> MLVEDLLKNNYLITPSAYYLLSDHYKKAFTLAELIKFAKNRGTFVVDSNLAREFLAEKGIISSGIVYGDYGVPIAYVADETPEEEKAYSTYSDLVIAPKEGFHYRAKEIPDEWELAFDVKNVKFEVPKVKNAQSKEGEVIIQAYSSYFKSRLKKMRRIFRENPEIGTIVDIAKLSYVREDDVTIIGLVNEKRETRKGYLFEIEDATGRIKVFIGSDKEGANEAYSTIMPDSVVAFRGTPGKGIFFANRVFLPDVPKFKRSKPPLEEKVYAILLSDIHVGSNKFCEEAFIKFLEWLNGEVNSRTEEELVSRIKYIIIGGDVVDGVGIYPGQYNELAIPDIFDQYEALANLLKQVPDHITMFIGPGNHDAARTALPQPGFYEEYAKPLYKLKNAVIISNPAVIRLHGRDFLVAHGRGIEDVVDFVPNRSHHRPAEAMVELLKLRHIAPTFGNKVPIAPDPEDTLVIESVPDLFQAGHVHVMQYKTYNGVFVINTGTWQAQTEFQKMVNIIPTPARVPIIDVETARLRAVVRFDQFCEGV;> MSEEIYSPEMKAYFESLQREIDRAYAIARKARAQGKDPSFDVEVPQATDMAGRVESLVGPPGVAERIRELVKEYGKEIAALKVVDEIIEGKFGDLGSKEKYAEQAVRTALAILTEGIVSAPLEGIADVKIKRNEWADGSEYLALYYAGPIRSSGGTAQALSVLVGDYVRRKLGLDRFKPSDEHIERMVEEVDLYHRAVTRLQYHPEADEVRLAMRNIPIEITGEETDKVEVSHRNVPGVETNHLRGGAILVLAEGVLQKAKKLVKYIDKMGIEGWDWIKEFVEAKEKGKSSEENKDESKAEDTGTESVAEKKENVEKGFYYELYEKFRANIAPNKKYTKEIIGGRPLFAEPSTNGGFRLRYGRSRVSGFATWSVNPATMLILDEFIAIGTQMKTERPGKGCIVTPATTVEGPIVRLKNGSVVRVDDYETALKVRNEVDEILYVGDALVNFGDFVENNQTLLPANYVEEWWVQELVQAIKDLYEVELQPFAENDREAVEEAAEYLEVDPDFLWNLLKDPLRVKPDVETAIHLSTVLDIPFHPYYTLYWNTLQPEEVEELQKALLGAQIEWAEFRKNRFAKKVVLENDKNIKRYLELLGLPHRLERVEKKRKVIVVEYPWSAALLTPLGNLEWEFKAKPFYTVIDIINENNRIKLRDRGISWIGARMGRPEKAKERKMKPPVQVLFPIGLAGGQSRDIKKAAEEGKTARVEIAFFKCPKCGHVGPEHLCPVCGTRKELLWHCPKCGADYPESDAKDFNYRCPKCDVELKPYAEREIKPADLLRQAMDNVKVYGIDRLKGVKGMTSGYKMAEPLEKGLLRVKNDVYVFKDGTIRFDATDAPITHFKPKEIGTSVEKLRELGYTHDFEGKPLERDDQILELKVQDVILPYEAGRYLLKVARFIDDLLEKFYGLPRFYNAEKMEDLVGHLVIGLAPHTSAGIIGRIIGFSDVLVGYAHPYYHAAKRRNCDGDEDAVMLLLDALLNFSKYYLPEKRGGKMDAPLVVTTRLDPREVDSEVHNMDVVRYYPLEFYKATYELKSPKEVKVIERVEDRLGKPEMYEGIKFTHDTDDIGLGPKMSLYKQLGDMEEKVARQLALAERIRAVDEHHVAETIINSHLVPDLRGNLRSFTRQEFRCVKCNTKYRRPPLTGKCPKCGGKIVLTVSKGAIEKYLPTAKMLVTKYRVKDYTRQRICITEKDIKTLFENVFPEKQRTLMGFSADICEKMVKERTGHSNGKNGYLDEFNGKNGKASKKSGSLASKLSGKGKEPSKKKESAKPKRSEKVKNLTSFEAAAKNEQARGTAGNAKKAESEKPKRKKRKGISLDEFFGS;>MPFEVVFDGAKEFADLIATASNLIDEAAFKFTEEGISMRAMDPSRVVLIDLNLPESIFSKYEVEEPETIGINMDQFKKILKRGKAKDTLILRKGDENFLEITFEGTAKRTFRLPLIDVEELELELPELPFTAKVVLLGEVLKEGIKDASLVSDAIKFIAKENEFTMKAEGETNEVEIRLTLEDEGLLDLEVEEETKSAYGIRYLSDMVKGIGKADEVILRFGNEMPLQMEYMIRDEGRLTFLLAPRVEE[3x]

PolD is the archaea-specific DNA polymerase that functions as the replicase in most of the organisms in Archaea except for Crenarchaeota. The PolD holoenzyme consists of two subunits, DP1 and DP2, which contain the catalytic sites of the 3′–5′ exonuclease and the 5′–3′ DNA polymerase, respectively. PCNA is the sliding clamp that enables high processivity of DNA polymerases and thus is an essential factor for replication. We obtained two structures, Form A and Form B, for the PolD-PCNA-DNA complex.

The DNA in Form B was bound to DP2 in a substantially different manner from that in Form A, and the orientation of the DNA bound to DP2 differs by 40° between the two forms. This swing motion appears to pull the growing end of the DNA out of the polymerase active site. Moreover, the nascent chain in Form B is unwound by five bases from the 3′-terminus. These results suggest that Form B corresponds to a state distinct from the synthesis mode and thus an editing mode. On the other hand, the DNA orientation is toward DP1, and the 3′-terminus of the DNA can reach the active center of the exonuclease in Form B, although the 3′-terminus was not observed in the EM structure. In the Form B complex, another contact was observed between PCNA and the central domain of DP2, due to the tilt of PolD. Intriguingly, the third glutamate, E171 (Fig. 5e: magenta sphere) of the PCNA trimer, not used in Form A, was involved in this PolD-PCNA contact. In contrast, PolD is substantially tilted on the PCNA in the Form B complex, and one of the three PCNA subunits is available to accept other factors. Therefore, exposure of one of the PCNA subunits in Form B appears advantageous for recruitment of additional PCNA-binding proteins to perform functions different from DNA synthesis.> GPLGSLCGRVFKVGEPTYSCRDCAVDPTCV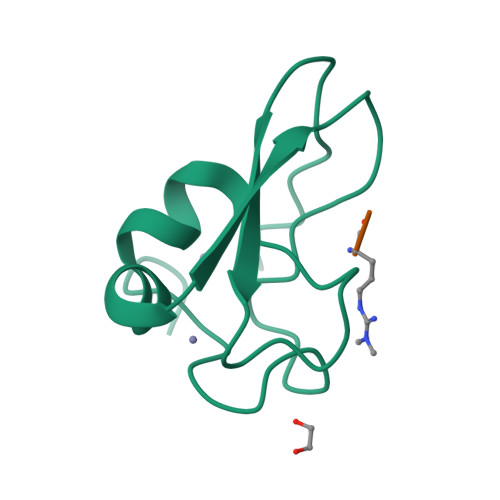LCMECFLGSIHRDHRYRMTTSGGGGFCDCGDTEAWKEGPYCQKHEL;> RIFS Another unicellular pappalysin is the T. forsythia KLIKK MP mirolysin, which protects the bacterium against complement-mediated bactericidal activity. It is secreted as a 66 kDa zymogen (see UniProt code A0A0F7IPS1), which when activated cleaves several physiologically relevant host proteins such as fibronectin; fibrinogen; complement proteins C3, C4 and C5; as well as antimicrobial peptide LL-37. As part of its virulence factor armamentarium, at the site of colonization it secretes mirolysin, a metallopeptidase of the unicellular pappalysin family, as a zymogen that is proteolytically auto-activated extracellularly at the Ser54–Arg55 bond. The catalytic domain conforms to the metzincin clan of metallopeptidases and contains a double calcium site, which acts as a calcium switch for activity.

A variant, in which the general base/acid Glu225 was replaced with alanine (E225A), lacked activity. This variant was used to obtain the intact zymogen for structural studies. Previously, this strategy has proven successful for other MP zymogens. We obtained two different crystal forms for native and selenomethionine-derivatized promirolysin E225A, which contained one and two protomers per asymmetric unit and diffracted to resolutions of 1.4 and 1.6 Å, respectively. Crystal structures of the catalytically impaired promirolysin point mutant E225A at 1.4 and 1.6 Å revealed that latency is exerted by an N-terminal 34-residue pro-segment that shields the front surface of the 274-residue catalytic domain, thus preventing substrate access. Promirolysin E225A has a compact structure of approximate dimensions 60 × 45 × 45 Å, and it splits into an N-terminal 34-residue PS (Arg21–Ser54) and a downstream 274-residue metzincin-type CD (Arg55–Leu328). Tyrosine-switch Tyr286 pinches the extended segment I together with the upper-rim-strand segment Leu181–Tyr183 of the CD. In the capital interaction for latency, downstream Cys23 Sγ binds the catalytic zinc at 2.11–2.22 Å in the different structures, which is closer than typical Zn–S distances (2.31 Å), and contributes together with the three histidine ligands to a tetrahedral zinc coordination sphere [Figs. 2(c) and 2(d)]. Finally, the primary activation site Ser54–Arg55 is access­ible, and Arg55 protrudes from the molecular surface by virtue of a hydrogen bond between Arg55 N and Asp308 Oδ2.

> GPQRTCGSELNMEQIRRTEPLKYQRITDWENQIKLHSRSVPSSTILIPVVVHVVYNNSAQNISDAQIISQIQVLNEDFRRMNADQANTPSAFANLAGNANIEFKLARRDPNGNTTNGITRTSTSTETFSMEMDNVKFSNLGGNNAWNTRRYLNIWVCNLGDDLLGYAQFPFEFQTKPNTDGVVIHYKHFGRDGSAESPYDKGRTATHAVGHWLDLRHIWGDDGGSCSGTDNIADTPNQGGYNEGCPSFPKTDHCTNTSPGVMFMNYMDYTYDACMNLFTKGQVERMRSLFDTQTGIRREMQIYANELTNPLSFS> RPEFDWQDPLVLEEQLTTDEILIRDTFRTYCQERLMPRILLANRNEVFHREIISEMGELGVLGPTIKGYGCAGVSSVAYGLLARELERVDSG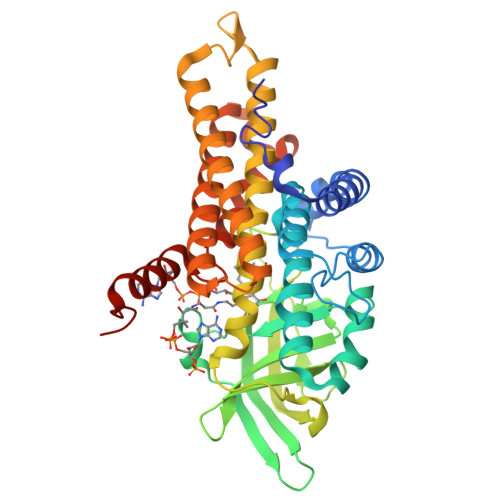YRSAMSVQSSLVMHPIYAYGSEEQRQKYLPQLAKGELLGCFGLTEPNSGSDPSSMETRAHYNSSNKSYTLNGTKTWITNSPMADLFVVWARCEDGCIRGFLLEKGMRGLSAPRIQGKFSLRASATGMIIMDGVEVPEENVLPGASSLGGPFGCLNNARYGIAWGVLGASEFCLHTARQYALDRMQFGVPLARNQLIQKKLADMLTEITLGLHACLQLGRLKDQDKAAPEMVSLLKRNNCGKALDIARQARDMLGGNGISDEYHVIRHAMNLEAVNTYEGTHDIHALILGRAITGIQAFTASK>[2x]GPSFWLGNETLKVPLALFALNRQRLCERLRKNPAVQAGSIVVLQGGEETQRY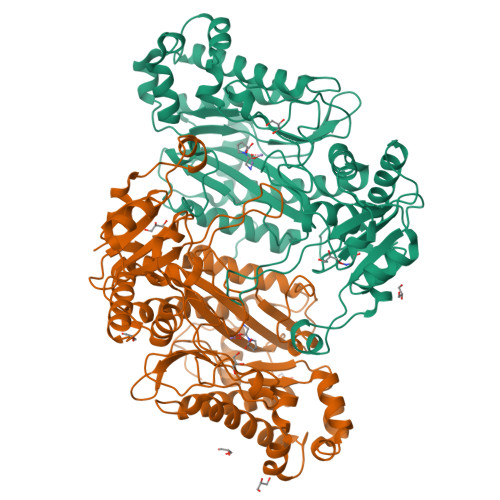CTDTGVLFRQESFFHWAFGVTEPGCYGVIDVDTGKSTLFVPRLPASHATWMGKIHSKEHFKEKYAVDDVQYVDEIASVLTSQKPSVLLTLRGVNTDSGSVCREASFDGISKFEVNNTILHPEIVECRVFKTDMELEVLRYTNKIFSEAHREVMKAVKVGMKEYELESLFEHYCYSRGGMRHSSYTCICGSGENSAVLHYGHAGAPNDRTIQNGDMCLFDMGGEYYCFASDITCSFPANGKFTADQKAVYEAVLRSSRAVMGAMKPGVWWPDMHRLADRIHLEELAHMGILSGSVDAMVQAHLGAVFMPHGLGHFLGIDVHDVGGYPEGVERIDEPGLRSLRTARHLQPGMVLTVEPGIYFIDHLLDEALADPARASFLNREVLQRFRGFGGVRIEEDVVVTDSGIELLTCVPRTVEEIEACMAGCDKAFTPF>GPLGSMSTPSLPIIDIAALAGSDPAARRSVAVRIDRACREQGFFYVVGHGVEAQLVERLERLARQFFALDETSKLRWRMELGGRAWRGYFPLGGELTSNRPDWKEGLYLGSELDAEHPEVRAGTPLHGANLFPEVPGLRETLLEYLDATTRVGHRLMEGIALGLGLEADYFAARYTGDPLILFRLFNYPSQPVPEGLDVQWGVGEHTDYGLLTLLHQDAIGGLQVRTPQGWLEAPPIPGSFVCNLGDMLERMTGGLYRSTPHRVARNTSGRDRLSFPLFFDPNFHARVQPIEGLPEVPEQDDSARRWDQANVHAFHGEYGD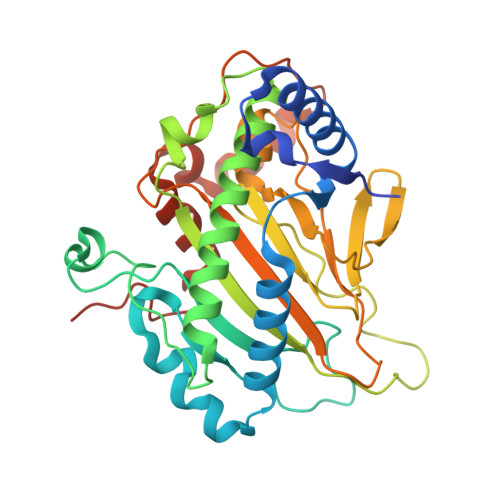YLLNKVAKVFPQLRRDLL[2x]>[2x]MGQEKLLFDQKYKIIKGEKKEKKKNQRANRREHQQKREIMRFKKSFTCIDMHTEGEAARIVTSGLPHIPGSNMAEKKAYLQENMDYLRRGIMLEPRGHDDMFGAFLFDPIEEGADLGIVFMDTGGYLNMCGHNSIAAVTAAVETGIVSVPAKATNVPVVLDTPAGLVRGTAHLQSGTESEVSNA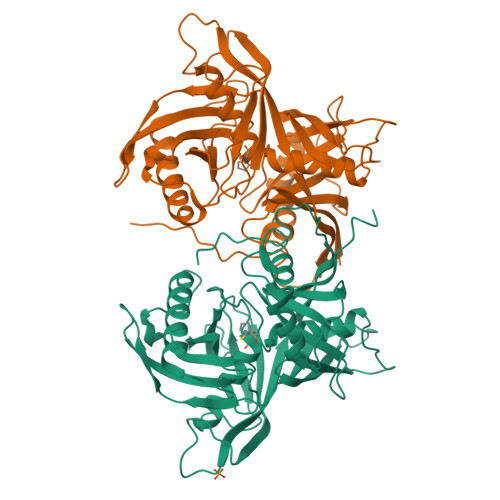SIINVPSFLYQQDVVVVLPKPYGEVRVDIAFGGNFFAIVPAEQLGIDISVQNLSRLQEAGELLRTEINRSVKVQHPQLPHINTVDCVEIYGPPTNPEANYKNVVIFGNRQADRSPCGTGTSAKMATLYAKGQLRIGETFVYESILGSLFQGRVLGEERIPGVKVPVTKDAEEGMLVVTAEITGKAFIMGFNTMLFDPTDPFKNGFTLKQYIWSSSVDKLAAALEHHHHHH> DPIHDRTSDYHKYLKVKQGDSDLFKLTVSDKRYIWYNPDPKERDSYECGEIVSETSDSFTFKTVDGQDRQVKKDDANQRNPIKFDGVEDMSELSYLNEPAVFHNLRVRYNQDLIYTYSGLFLVAVNPFKIIPIYTQEMVDIFKGRRRNEVAPHIFAISDVAYRSMLDDRQNQSLLITGESGAGKTENTKKVIQYLASVAGRNQANGSGVLEQQILQANPILEAFGN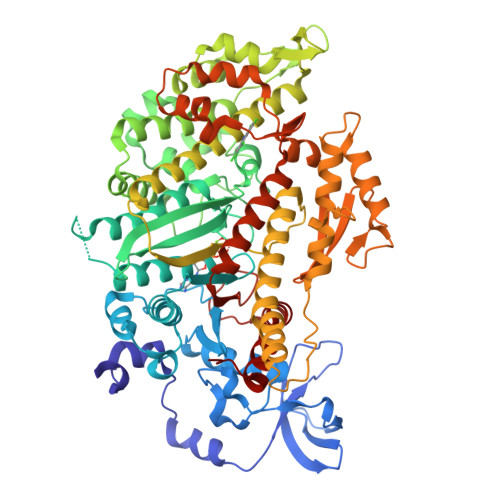AKTTRNNNSSRFGKFIEIQFNSAGFISGASIQSYLLEKSRVVFQSETERNYHIFYQLLAGATAEEKKALHLAGPESFNYLNQSGCVDIKGVSDSEEFKITRQAMDIVGFSQEEQMSIFKIIAGILHLGNIKFEKGAGEGAVLKDKTALNAASTVFGVNPSVLEKALMEPRILAGRDLVAQHLNVEKSSSSRDALVKALYGRLFLWLVIKINNVLCQERKAYFIGVLDISGFEIFKVNSFEQLCINYTNEKLQQFFNHHMFKLEQEEYLKEKINWTFIDFGLDSQATIDLIDGRQPPGILALLDEQSVFPNATDNTLITKLHSHFSKKNAKYEEPRFSKTEFGVTHYAGQVMYEIQDWLEKNKDPLQQDLELCFKDSSDNVVTKLFNDPNIASRAKKGANFITVAAQYKEQLASLMATLETTNPHFVRCIIPNNKQLPAKLEDKVVLDQLRCNGVLEGIRITRKGFPNRI> AAQTNAPWGLARISSTSPGTSTYYYDESAGQGSCVYVIDTGIEASHPEFEGRAQ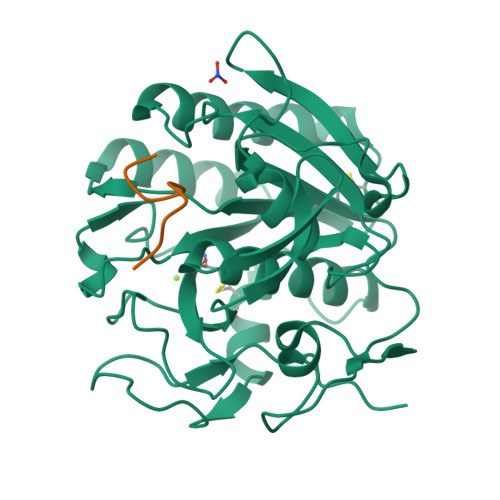MVKTYYYSSRDGNGHGTHCAGTVGSRTYGVAKKTQLFGVKVLDDNGSGQYSTIIAGMDFVASDKNNRNCPKGVVASLSLGGGYSSSVNSAAARLQSSGVMVAVAAGNNNADARNYSPASEPSVCTVGASDRYDRRSSFSNYGSVLDIFGPGTDILSTWIGGSTRSISGTSMATPHVAGLAAYLMTLGKTTAASACRYIADTANKGDLSNIPFGTVNLLAYNNYQA;> KGEADALSLD> DNSRYTHFLTQHYDAKPQGRDDRYCESIMRRRGLTSP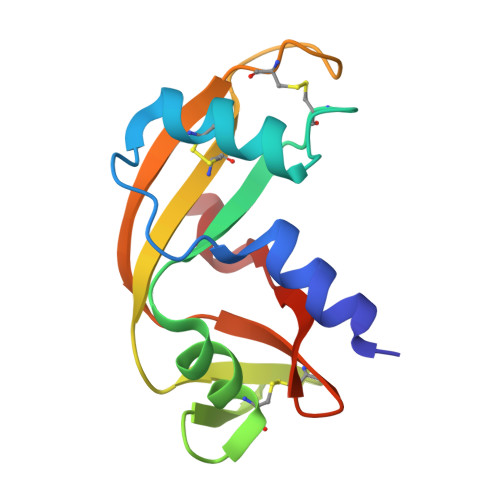CKDINTFIHGNKRSIKAICENKNGNPHRENLRISKSSFQVTTCKLHGGSPWPPCQYRATAGFRNVVVACENGLPVHLDQSIFRR3-(3-benzyl-2-oxo-2H-[1,2,4]triazino[2,3-c]quinazolin-6-yl)propanoic 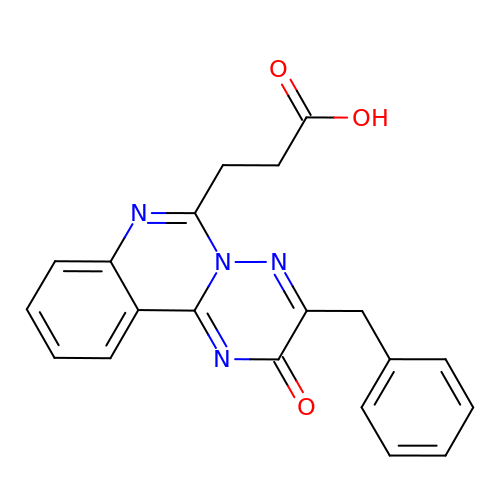acid | C20 H16 N4 O3 | RRZGYLKTEQRDCA-UHFFFAOYSA-N> 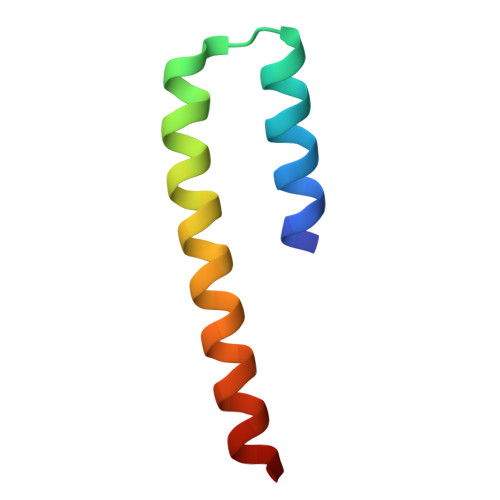XCLAALRSELQALRREGFSPEELAALESELQALERELAALRSELQALRGX>GPHTGGIMISSTGEVRVDNGSFHSDVDVSAVTTQAEAGFLRARGTIISKSPKDQRLQYKFTWYDINGATVEDEGVSWKSLKLHGKQQ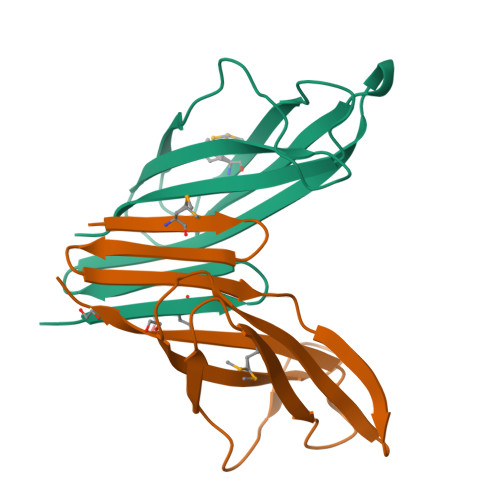MQVTALSPNATAVRCELYVREAISN[2x]>MRVLVINSGSSSIKYQLIEMEGEKVLCKGIAERIGIEGSRLVHRVGDEKHVIERELPDHEEALKLILNTLVDEKLGVIKDLKEIDAVGHRVVHGGERFKESVLVDEEVLKAIEEVSPLAPLHNPANLMGIKAAMKLLPGVPNVAVFDTAFHQTIPQKAYLYAIPYEYYEKYKIRRYGFHGTSHRYVSKRAAEILGKKLEELKIITCHIGNGASVAAVKYGKCVDTSMGFTPLEGLVMGTRSGDLDPAIPFFIMEKEGISPQEMYDILNKKSGVYGLSKGFSSDMRDIEEAALKG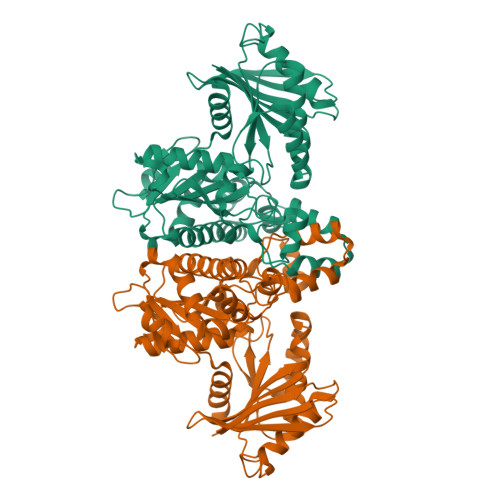DEWCKLVLEIYDYRIAKYIGAYAAAMNGVDAIVFTAGVGENSPITREDVCSYLEFLGVKLDKQKNEETIRGKEGIISTPDSRVKVLVVPTNEELMIARDTKEIVEKIGR[10x]>GAMGDQKPIGVAVLGLGNVGSEVVRIIDESATDLAARIGAPLQLRGIGVRRVSADRGVPVELLTDNIEELVSRDDVDIVVELMGPVEPARKAILTALEQGKSVVTANKALMSVSTGELAQAAEAAHVDLYFEAAVAGAIPVIRPLTQSLAGDTVTRVAGIVNGTTNYILSAMDSTGADYGDALAEASALGYAEADPTADVEGYDAAAKAAILASIAFHTRVTADDVYREGITKVTAADFASARALGCTIKLLAICERLTSDDGHQSVSARVYPALVPLTHPLAAVNGAFNAVVVEAEAAGRLMFYGQGAGGAPTASAVMGDVVMAARNRVQGGRGPRESKYAKLPISPIGDIPTRYYVSMRVADRPGVLAAVATEFGNRSVSIAEVRQEGIDD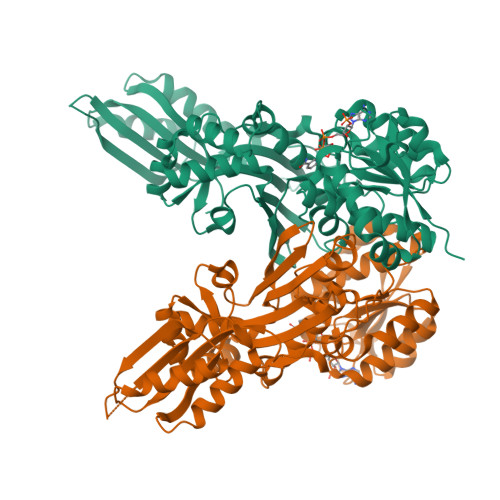GGEPRGARLVVVTHKATDAALSETVKALASLDVVQSVDSVIRMEGTSE[4x]>SNASAEDVLNLLRQAHEQEVFDADTLLRLEKVLDFSDLEVRDAMITRSRMNVLKENDSIERITAYVIDTAHSRFPVIGEDKDEVLGILHAKDLLKYMFNPEQFHLKSILRPAVFVPEGKSL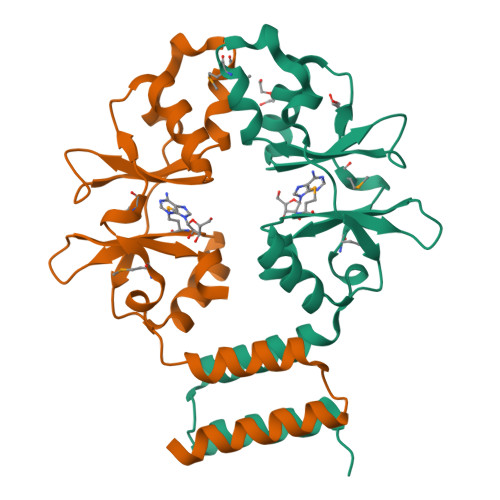TALLKEFREQRNHMAIVIDEYGGTSGLVTFEDIIE[2x]>[4x]MGSSHHHHHHGSGGGNNNNNNNNNNLGIEENLYFQSHMMKFTIQKDRLVESVQDVL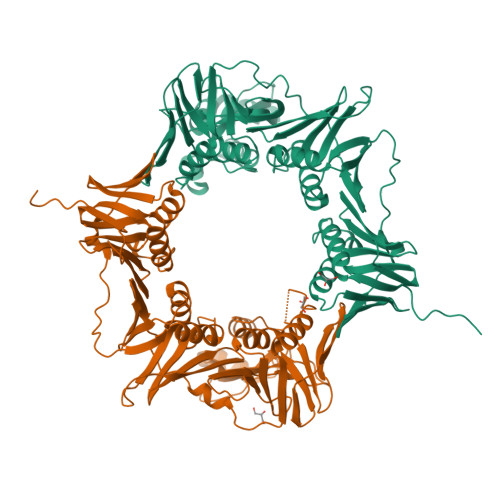KAVSSRTTIPILTGIKIVASDDGVSFTGSDSDISIESFIPKEEGDKEIVTIEQPGSIVLQARFFSEIVKKLPMATVEIEVQNQYLTIIRSGKAEFNLNGLDADEYPHLPQIEEHHAIQIPTDLLKNLIRQTVFAVSTSETRPILTGVNWKVEQSELLCTATDSHRLALRKAKLDIPEDRSYNVVIPGKSLTELSKILDDNQELVDIVITETQVLFKAKNVLFFSRLLDGNYPDTTSLIPQDSKTEIIVNTKEFLQAIDRASLLAREGRNNVVKLSAKPAESIEISSNSPEIGKVVEAIVADQIEGEELNISFSPKYMLDALKVLEGAEIRVSFTGAMRPFLIRTPNDETIVQLILPVRTYVDSVEPEVQEMIVPLTFHYSTNEALIIEQHKQELESVGVFLESFGSNSYIVRCHPAWFPKGEEAELIEEIIQQVLDSKNIDIKKLREEAAIMMSCK> MTTVVSRTFRSSPHRDALQTWDAIVELLTQGKDGTARSELRAVTGVAASLIA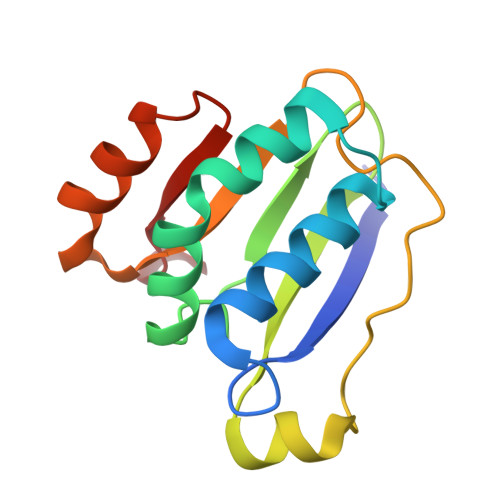DQAPKSAPIVATCDGPRTRIYCLFDEDAIDGDDANEEVLGFEPLKGDWGVSLPCPKEQLGWVQSALKKHSSRIIARDLSQG N-{[(2R,3R,4R,5R,6S)-3,4,5-trihydroxy-6-methylpiperidin-2-yl]methyl}acetamide 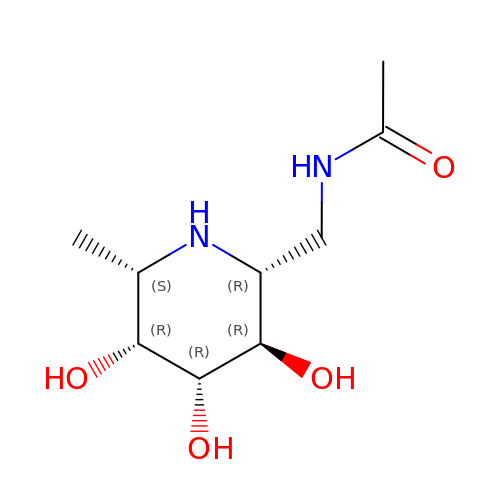| C9 H18 N2 O4 | PCXCXTZASITUBF-GDJKBKKHSA-N> GYGEVLVPE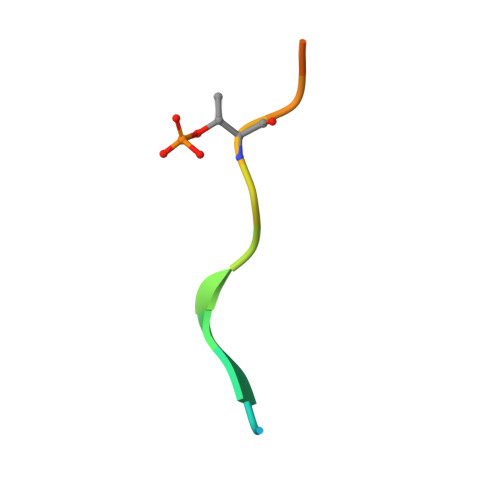TVAQHRT>AAPLEGRNVAIASPNAIVRAATARQIEAAGGRAYAAVDIASALAGAPADAVLLIDAALSGPRGALKPPAGRRSVVLLTPEQRDRIDRLKAAGFSGYLIKPLRAASLVA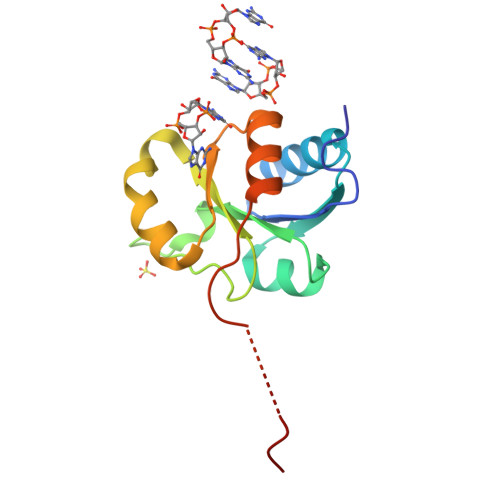QVLQAVTADGVAEDEPAHDDRI[2x]> MTRLLVLGGTTEASRLAKQDADQGFEAVFSYAGRTGAPVAQPLPTRIGGFGGVAGLVDYLTREGVSHVIDATHPFAAQMSANAVAACAQTGVALCAFERAPWTAQAGDRWTHVPDLAAAVAALPQAPARVFLAIGKQHLRDFSAAPQHHYLLRLVDPPEGPLPVPDARAVIARGPFTVQGDTELLRSETITH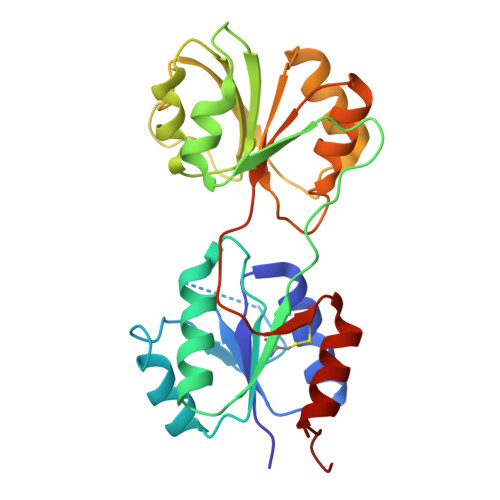VVAKNAGGAGAEAKLIAARSLGLPVILIDRPAVPARDICATLEGVMGWLADHGATPRGV> ALETLAFDGRTYIEYLNAVIESELTNEIPAEKALQSNHFELSLRTEATQGLVLWIGKAAERADYMALAIVDGHLQLSYDLGSQPVVLRSTVKVNTNRWLRIR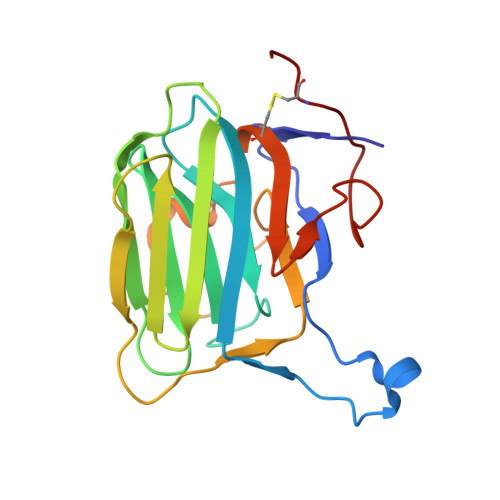AHREHREGSLQVGNEAPVTGSSPLGATQLDTDGALWLGGLQKLPVGQALPKAYGTGFVGCLRDVVVGHRQLHLLEDAVTKPELRPCPTP>[3x]MRGSHHHHHHGSMKTVLCYGDSLTWGYDATGSGRHALEDRWPSVLQKALGSDAHVIAEGLNGRTTAYDDHLADCDRNGARVLPTVLHTHAPLDLIVFMLG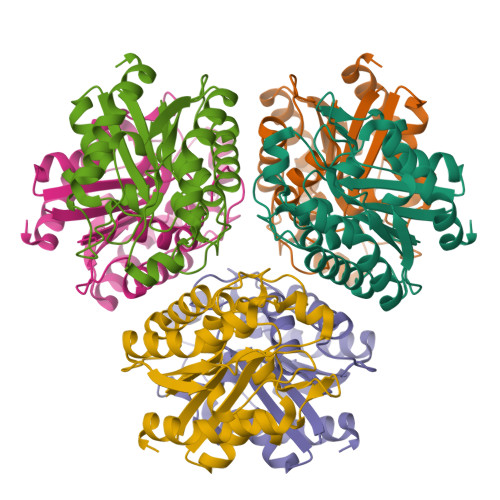SNDMKPIIHGTAFGAVKGIERLVNLVRRHDWPTETEEGPEILIVSPPPLCETANSAFAAMFAGGVEQSAMLAPLYRDLADELDCGFFDGGSVARTTPIDGVHLDAENTRAVGRGLEPVVRMMLGL>GQPPPIQLATNYRQDIDVTQYYVSEKLDGIRAYWNGHQLISKQGNIFTAPTWFIASFPTTAMDGELWIARQQFETVSGIARTQDNQNEQWKQIKFMIFDLPKSTVSFEQRINKMQTLVTDTNSPYLQMIEQQKIPNTVALFDLLNKVVMGKGEGLMLHHQDALYQTKRSRDLMKLKKFEDAEATVIAYLPGKGKYEGLLGAILVKNEEGVTFKIGSGFSDEERSTPPPIGSLITYRFTGKTNNNIPRFASFVRIRVIY[2x]

DNA ligases are a structurally diverse class of enzymes which share a common catalytic core and seal breaks in the phosphodiester backbone of double-stranded DNA via an adenylated intermediate. The sealing of breaks in the phosphodiester backbone of double-stranded DNA is essential for the replication and survival of all organisms. This function is carried out by DNA ligases in a three-step reaction in which the enzyme first self-adenylates, followed by DNA binding and transfer of AMP to the 5′-phosphate terminus of the DNA nick, which is then activated for nucleophilic attack by the apposing 3′-OH group. ATP-dependent DNA ligases (abbreviated ADLs) share a common catalytic core which includes all six of the conserved nucleotidyltransferase motifs and comprises the adenylation domain (AD domain), where the AMP cofactor is covalently bound, and an oligonucleotide-binding domain (OB domain), which engages the minor groove of the DNA duplex upon nick binding and assists in the step 1 adenylation reaction. Here, we report the biochemical and structural characterization of a bacterial ADL present in the partially sequenced genome of the psychrotolerant Psychromonas sp. strain SP041 isolated from Svalbard, Norway. This protein, hereafter referred to as Psy-Lig, is a minimal type of bacterial ADL possessing only the catalytic domains necessary for self-adenylation and nick-sealing and an N-terminal periplasmic localization sequence.

The 1.65 Å resolution structure of the enzyme–adenylate complex presented here represents only the second structure of a bacterial ADL to date and is the only available structure of the minimal type of bacterial ADL. Each Psy-Lig monomer has a large (172-residue) N-terminal AD domain comprising two four-stranded β-sheets surrounded by five α-helices and a smaller (77-residue) OB domain comprising a five-stranded β-barrel and a single α-helix. The two domains are connected by an eight-residue linker, and in both Psy-Lig chains these adopted the open conformation typical of the enzyme–adenylate intermediate, in which the DNA-binding surfaces of the two domains face away from each other. AMP bound in the active site was clear in the observed electron density, covalently linked to Lys25 via a phosphoamide bond to the side-chain Nζ atom, which is consistent with exposure of the protein to high levels of ATP during purification. As in other ligase–adenylate structures, the AMP is in the anti conformation, with the adenine nucleotide base stacked between the hydrophobic side chains of Phe97 in motif IIIa and Met155 in motif IV. Nine sulfate molecules were also resolved in the electron density, one of which is located in the active site of chain A. A sulfate ion at the equivalent position in ChlV-Lig–AMP occupies the binding site of the nicked 5′ DNA in ChlV-Lig–DNA, a structure which is also likely to be the case here.>[4x]MGSSHHHHHHGSLPPREDAARVARFVTHVSDWGALATISTLEAVRGRPFADVLSLSDGPPGAGSGVPYFYLSPLQLSVSNLQENPYATLTMTLAQTNFCKKHGFD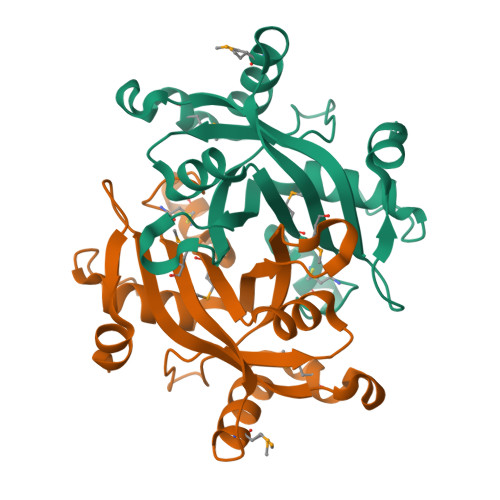PQSPLCVHIMLSGTVTKVNETEMDIAKHSLFIRHPEMKTWPSSHNWFFAKLNITNIWVLDYFGGPKIVTPEEYYNVTVQ>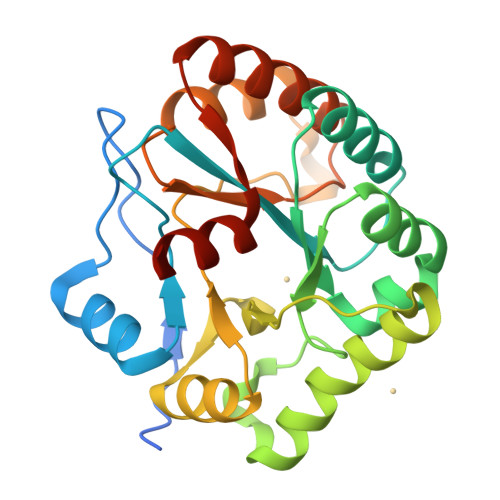[2x]GPLGSVLLAGGAAQAEAVPNEPINWGFKRSVNHQPPDAGKQLNSLIEKYDAFYLGNTKEKTIYLTFDNGYENGYTPKVLDVLKKHRVTGTFFVTGHFVKDQPQLIKRMSDEGHIIGNHSFHHPDLTTKTADQIQDELDSVNEEVYKITGKQDNLYLRPPRGVFSEYVLKETKRLGYQTVFWSVAFVDWKINNQKGKKYAYDHMIKQAHPGAIYLLHTVSRDNAEALDDAITDLKKQGYTFKSIDDLMFEKEMRLPSL>GHMSTTARFDSIGGLFEDFTQSAAQRAIEVRTIFHMIGDVSGKSVLDLACGFGFFGREIYRRGAAKVVGVDISEKMIELAREESRKYGDPLEFHVRDVANMEPLGQFDLVNAAWLFNYADSVENLRKMFKVVRASLKPDGKLVAYTVDPDFSLAKGNFAK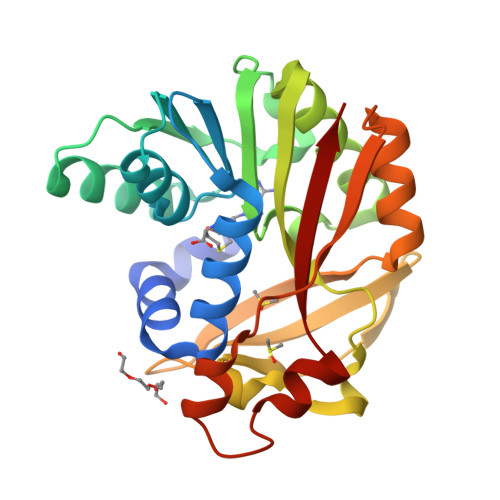YGVNVLNERAWGPGYRHDAEFVTDPPSQFSFYRWSRADYESAIADAGFSHFEWQKPLLEADDIATHPPGFWDVFQNNCLQTGLVCKP[2x]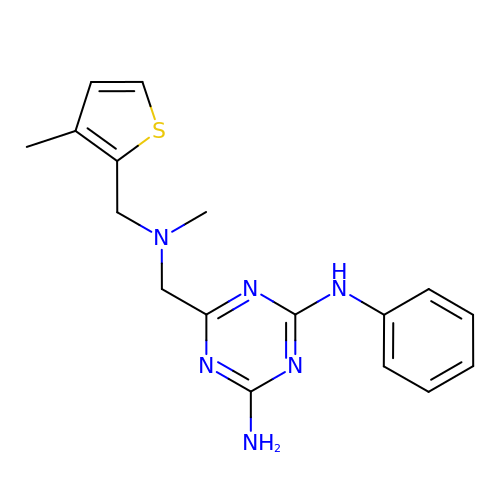6-[[methyl-[(3-methylthiophen-2-yl)methyl]amino]methyl]-~{N}4-phenyl-1,3,5-triazine-2,4-diamine | C17 H20 N6 S | PJORKXLDJATLJK-UHFFFAOYSA-N> MSGIALSRLAQERKAWRKDHPFGFVAVPTKNPDGTMNLMNWECAIPGKKGTPWEGGLFKLRMLFKDDYPSSPPKCKFEPPLFHPNVYPSGTVCLSILEEDKDWRPAITIKQILLGIQELLNEPNIQDPAQAEAYTIYCQNRVEYEKRVRAQAKKFAPS;> NNDHINLKVAGQDGSVVQFKIKRHTPLSKLMKAYCERQGLSMRQIRFRFDGQPINETDTPA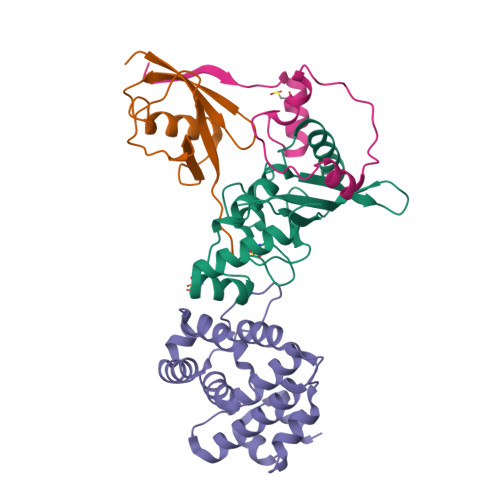QLEMEDEDTIDVFQQQTGG;> SLTGEPAPVLSSPPPADVSTFLAFPSPEKLLRLGPKSSVLIAQQTDTSDPEKVVSAFLKVSSVFKDEATVRMAVQDAVDALMQKAFNSSSFNSNTFLTRLLVHMGLLKSEDKVKAIANLYGPLMALNHMVQQDYFPKALAPLLLAFVTKPNSALESCSFARHSLLQTLYKV;> SLDVLIVYELTPTVEEKAKADTLKLPPTFFCYKNRPDYVSEEEEDDEDFETAVKKLNGKLYLDGSEK> SLMVPVEIRWQQGGSKVYVTGSFTKWRKMIGLIPDSDNNGSFHVKLRLLPGTHRFRFIVDNELRVSDFLPTATDQMGNFVNYIEVRQPEKNPTNEKIRSKEADSMRPPTSDRSSIALQIGKDPDDFGDG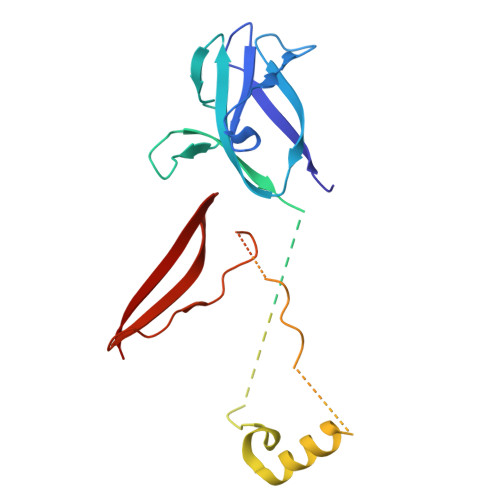YTRFHEDLSPRPPLEYTTDIPAVFTDPSVMERYYYTLDRQQSNTDTSWLTPPQLPPQLENVILNKYYATQDQFNENNSGALPIPNHVVLNHLVTSSIKHNTLCVASIVRYKQKYVTQILYTPI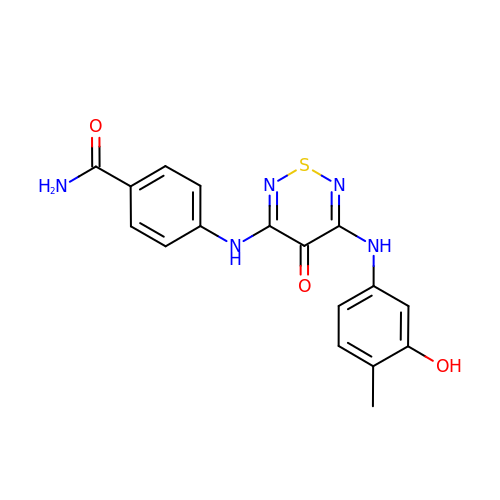4-({5-[(3-hydroxy-4-methylphenyl)amino]-4-oxo-4H-1,2,6-thiadiazin-3-yl}amino)benzamide | C17 H15 N5 O3 S | DHBUOVPLOHMOJE-UHFFFAOYSA-N> MDVASSDTVYTFPDEFKLGAATASYQIEGAWDENGKGPNIWDTLTHEHPDYVVDGATGDIADDSYHLYKEDVKILKELGAQVYRFSISWARVLPEGHDNI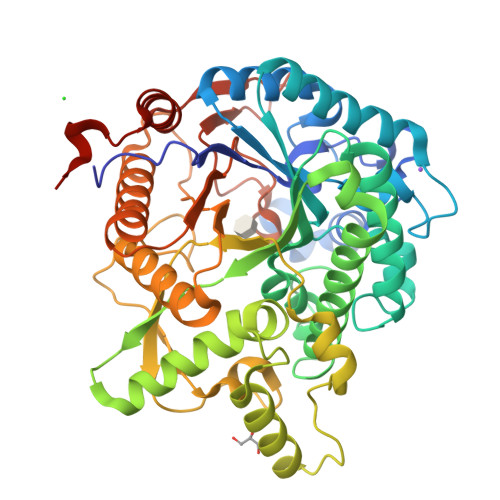VNQDGIDYYNNLINELLANGIEPMVTMYHWDLPQALQDLGGWPNLVLAKYSENYARVLFKNFGDRVKLWLTFNDPLTFMDGYASEIGMAPSINTPGIGDYLAAHTVIHAHARIYHLYDQEFRAEQGGKVGISLNINWCEPATNSAEDRASCENYQQFNLGLYAHPIFTEEGDYPAVLKDRVSRNSADEGYTDSRLPQFTAEEVEYIRGTHDFLGINFYTALLGKSGVEGYEPSRYRDSGVILTQDAAWPISASSWLKVVPWGFRKELNWIKNEYNNPPVFITENGFSDYGGLNDTGRVHYYTEHLKEMLKAIHEDGVNVIGYTAWSLMDNFEWLRGYSEKFGIYAVDFEDPARPRIPKESAKVLAEIMNTRKIPERFRDLEHHHHHH> MNIVLMGLPGAGKGTQAERIVEKYGIPHISTGDMFRAAM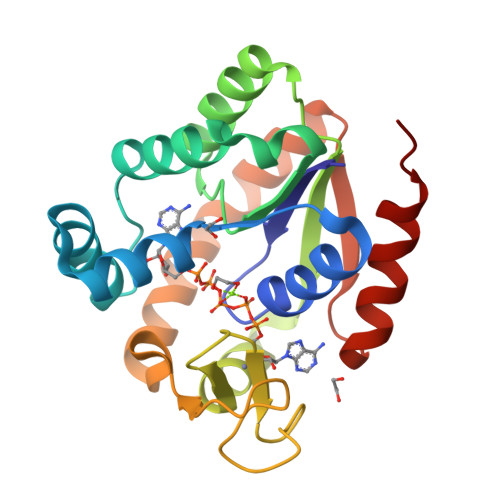KEETPLGLEAKSYIDKGELVPDEVTIGIVRERLSKSDCERGFLLDGFPRTVAQAEALEEILEEMGRPIDYVINIQVDKEELMERLTGRRICSVCGTTYHLVFNPPKTPGICDKDGGELYQRADDNEETVTKRLEVNMKQTAPLLAFYDSKEVLVNVNGQQDIQDVFADVKVILGGLKQ Replication initiator proteins (Reps) from the HUH-endonuclease superfamily process specific single-stranded DNA (ssDNA) sequences to initiate rolling circle/hairpin replication in viruses, such as crop ravaging geminiviruses and human disease causing parvoviruses. At the heart of DNA processing of all HUH-endonucleases is a structurally defined catalytic nickase domain that first recognizes a specific sequence/structure of DNA; nicks ssDNA at a ‘nic site’ to yield a sequestered 5′ end that remains covalently bound to the HUH endonuclease and a free 3′OH that can be used as a primer for DNA replication; and finally, facilitates a strand transfer reaction to resolve the covalent intermediate. To uncover the ssDNA recognition mechanism of Reps and identify potential motifs that might confer sequence specificity, we solved the first high resolution crystal structures of two Rep nickase domains from Porcine circovirus 2 (PCV2) and Wheat dwarf virus (WDV) with 12% sequence identity, bound to ssDNA encoding minimal sequences comprising the respective origin of replication (ori) sequences. With this, we term this turn-β-turn structural motif as the ‘single-stranded DNA Bridging Motif’ (sDBM), and suggest that it is the main binding moiety responsible for recognition and conformation priming of ssDNA by Rep HUH-endonucleases.

We present structures of two 10-mer bound structures of inactive PCV2Y96F (1.93 Å resolution) and WDVY106F (1.80 Å resolution), and one 8-mer bound WDVY106F (2.61 Å resolution) structure. The pre-cleavage state was captured by mutating the catalytic tyrosine to phenylalanine. All three structures are in complex with the divalent cofactor manganese. Additionally, the catalytic tyrosine (though a Phe mutant in the structures) is positioned for nucleophilic attack of the scissile phosphate, where the active oxygen of PCV2 and WDV is measured at 2.2 and 2.9 Å from the phosphate, respectively. Strikingly, despite the absence of bases that make up the hairpin stem in the short target DNA oligos, the ssDNA is bent into a ‘U-shaped’ architecture like one might expect in the context of the hairpin loop. The U-shaped DNA sits in a shallow channel on the surface of one face of the Rep protein with a distinct topological ‘nose’ that juts out in the center of the U. The bent conformation of the ssDNA in the Rep structures is driven by both intermolecular interactions with the topological ‘nose’ of the protein and by intramolecular Watson–Crick base pairing between T−4 and A+1 along with adjacent hydrogen bonding between N3 of T−1 and N3 of A−3. The consecutive stretch of 9–10 residues in the turn-β4-turn structural motif (‘ARCHIEKAKG’ for PCV2 and ‘HPNIQAAKD’ for WDV) has two critical functions in the structure. First, it acts as a ‘bridge’ between 5′ and 3′ ends of the nonanucleotide sequence contacting positions −6, −5, +1 and +2.

>[3x]PSKKNGRSGPQPHKRWVFTLNNPSEDERKKIRDLPISLFDYFIVGEEGNEEGRTPHLQGFANFVKKQTFNKVKWYLGARCHIEKAKGTDQQNKEFCSKEGNLLMECGAPRSQGQR> MFHLVDFQVTIAEILLIIMRTFKVSIWNLDYII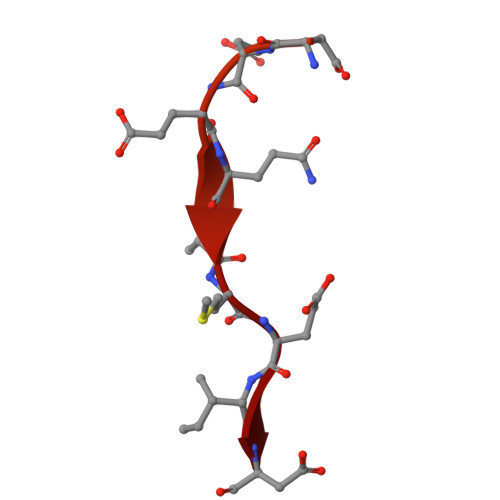NLIIKNLSKSLTENKYSQLDEEQPMEID> MASIPSAAPSWRKMQIPRPLQRLFDYFPLRIYEPNELPERSQQLTSGDLPTLYVFSTDSDARLGLPSFNPGCLKWQTLLRLANLDFRILPSTNHS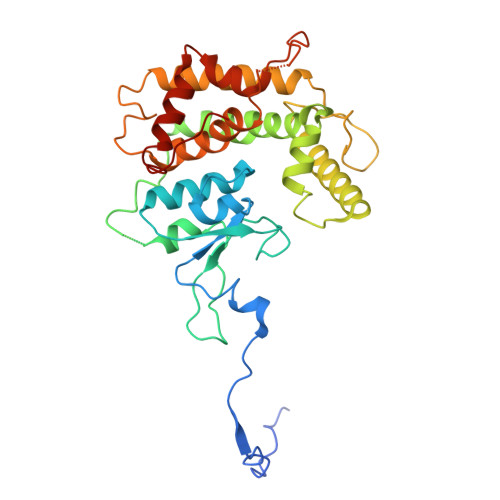SPTGSLPFLLPPRTSPTASPAPIPASGLLSFARKNPWRPGKAADLDLGHLDADLPPRAQAYLALITHSLRNAWLCALYLDPTHDALLRRLYVDPASSSRAVRAALLHQLRRAAAEQVATASSGGGKIVSLAPVDSADGIDEEAVYRSARDALDALASLLRESETAWFFGTERPGSFDAALFSYTHLMVEYMSEEEDTESAKGRVSLGRMVKEAGNGELAEHRERMLGVAWPEWDGYRR> RRVRK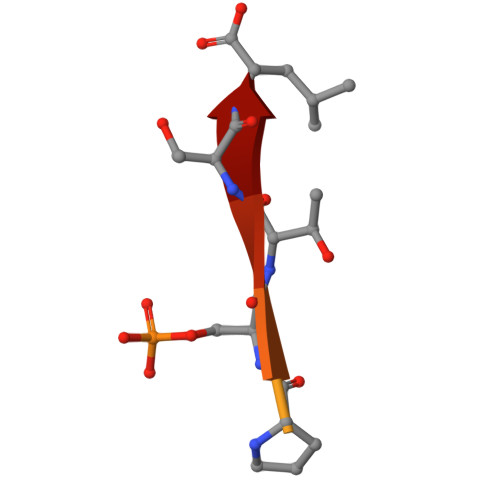LPSTTL>[6x]MSAKKTNEKRSEIQSETNTTSLDEVADIELEFEKADVELLKHQVELFNPLYEKRAMVLRKIPKFWPIAIEAAPSDELSVYISPEDANVLEHLIDLRVYRPNEDPRDIKIVFEFEANEYLESNSLYLMKLFRYSSQKAEASSSNINKEPSQLISEKVNIEWKKNKDLTRQTKGTAPSFFTWFSWTGKENDIFEDEEELAIFIAEDLYPNAVKYFTDALQENEENEDEEIDLENENGDNISEEEPSKKRTKL

Sequence alignment revealed that Vps75 is a member of the evolutionarily conserved nucleosome assembly protein 1/SE translocation (NAP1/SET) superfamily, members of which function as escorts for histone (H3–H4)2 tetramers and H2A–H2B dimers. Two histone chaperones, Vacuolar Protein Sorting 75 (Vps75) and the Anti-Silencing Function 1 protein (Asf1), are involved in the Rtt109-dependent histone H3K9, H3K27, and H3K56 acetylation. In this study, we solved both dimeric and tetrameric structures of Vps75 from a pathogenic fungus, P. carinii (PcVps75), and identified a structural basis for the inability of PcVps75 to interact with PcRtt109. Therefore, we propose that Vps75 regulates the HAT activity of Rtt109 by affecting the interactions between histones and specific histone chaperones rather than by forming a complex with Rtt109.

The PcVps75 tetramer consists of two identical PcVps75 dimers, dimer I: A/B (orange and yellow) and dimer II: C/D (green and dark green). Four quasi-equivalent protomers of PcVps75 are arranged in a solid, walnut-like structure. Two parallel α-helices (αA1/αB1, αC1/αD1) are present on each side of the PcVps75 tetrameric core, which is composed of four domain IIs. Within the core interior, each PcVps75 dimer contributes two domain IIs, including α-helices (α2–α8) and β–sheets (β1–β3), to form a golf ball-like structure. In this area, residues Y80, F177, W180, and L197 on loop LP1A of protomer A form a hydrophobic interface that surrounds the highly conserved residue F191 on loop LP2D from the opposite PcVps75 protomer D. The polyanion clusters binding to Ca2+ in the Vps75 tetramer neutralize the negative electric charge on the concave surfaces of the PcVps75 dimer, making it more convenient to cover two dimeric PcVps75s together in a tetrameric form. In the PcVps75 tetramer, residues E192, D193, E194, and E196 were involved in a calcium-binding cluster that had essential roles in sustaining the PcVps75 tetramer by burying histone-binding surfaces within the structure. The PcVps75 tetramer conceals the major histone-binding surface of PcVps75, which may be a way of preventing non-specific interactions. When tetrameric PcVps75 encounters histones, it can dissociate into two PcVps75 dimers, thereby exposing the histone-binding surfaces to the histone cargo.>MSANVQEAANAAIEPASFVKVPMPEPPSSLQQLINDWQLIKHREGGYFKETDRSPYTMEVEKPVNGGSGNTEMVTRNQSTLIYYLLTPDSPIGKFHKNINRIIHILQRGKGQYVLVYPDGQVKSFKVGFDYKNGEVSQWVVPGGVFKASFLLPNEEFDNGFLISEV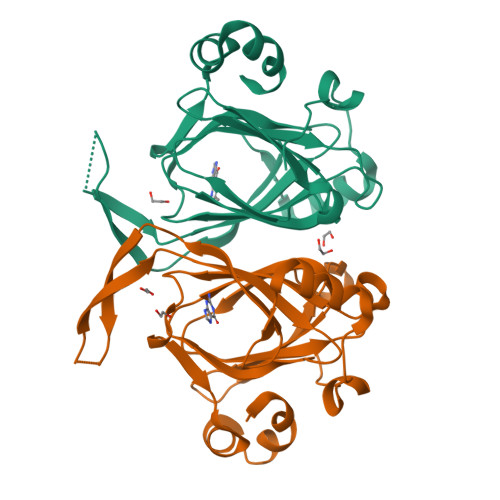VVPGFDFEDHTFLKGEDELKHLVGPEKAAELAFLAHH[3x]>MVEYHIPSWDEIEDAVFSIGEALVKSNYIPDVLIAVLTGGIIPAKLLSDLLDLKVIRYIDIKFYRS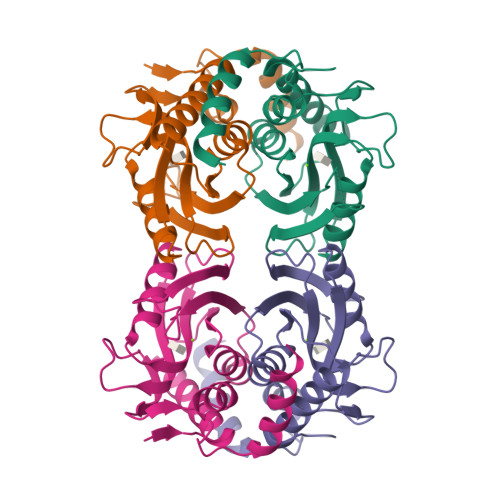VGKTESKPVIRSVYTDSLEGKKVLVVDDVADTGETLEAVSNVITMFNPAKVMTAALYLKPWSKRIPDFYYKQIDKWIIFPWDKWDVVRENSNVPVDKKERFLNLYNQLLKIRK[2x]>MSFTVDSARGIFPNTLTADVVPATIARFNQLNAEDQLALIWFAYLEMGKTITVAALGAANMQFAEITMNQIRQMSFQEQTQVMCDLANRTDTPISRAYGSWTANIKLGFWYQLGEWMAQGIVAPIPSGYKLSANAASVLQAIQGLESGQQITVLRNCVVDMGFDTSKLDSSQRVSEPVVVPRDMAQRTQVTIEGIDNPTVLNYMNNMNANDFEVLIELFTPDGALQPPFQKPIVGKDAVLRFFREECQNLKLIPERGVTEPADGGYTQIKVTGKVQTPWFGAGVGMNMAWRFLLSPENKIFFVAID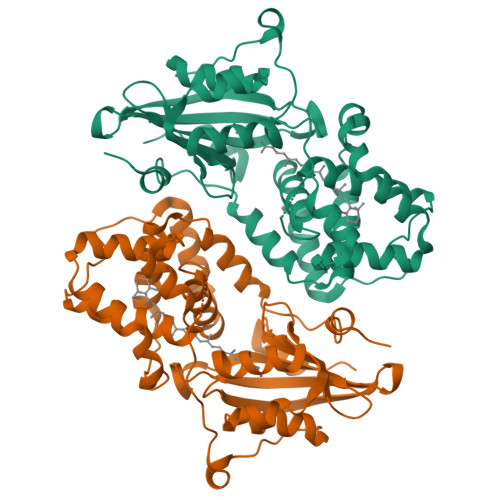LLASPKELLNLVR[2x]>[10x]MLYLVRMTVNLPRNLDPREEERLKASEKA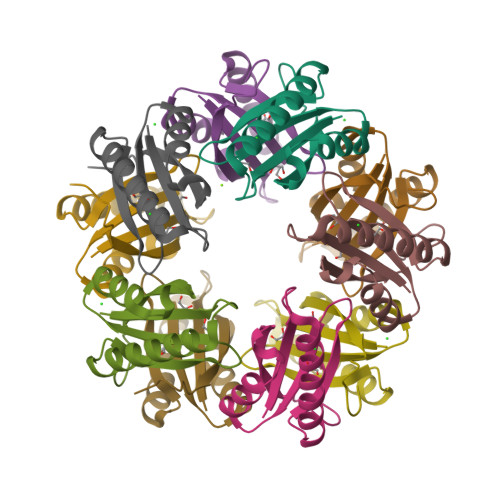RSRTLQEQGQWRYLWRTTGKYGNISVFDVNSHDELHEILWSLPFFPYLTIDVEPLSHHPARVGKD>MSCGNAKINSPAPSFEEVALMPNGSFKKISLSSYKGKWVVLFFYPLDFTFVCPTEVIAFSDSVSRFNELNCEVLACSIDSEYAHLQWTLQDRKKGGLGTMAIPILADKTKNIARSYGVLEESQGVAYRGLFIIDPHGMLRQITVNDMPVGRSVEEVLRLLEAFQFVEKHGEVCPANWKKGDPGMKPEPNASVEGYFSKQ[5x]

T(SH)2 participates in crucial thiol-disulfide exchange reactions and serves as electron donor in the reduction of hydrogen peroxide to water catalyzed by the tryparedoxin/tryparedoxin peroxidase couple (TXN/TXNPx). Leishmania major TXNPx (LmTXNPx) is an obligate homodimer whose active site is formed by the N-proximal peroxidatic cysteine (Cp) from one subunit and a C-proximal resolving cysteine from the two-fold symmetry related subunit (Cr′)89. In the first reaction, oxidized TXNPx binds TXN, which reduces the inter-subunit disulfide bridge (Cp–Cr′) and, thereafter, is reduced by T(SH)2. In the second reaction, the Cp thiolate of a TXNPx monomer reduces the hydrogen peroxide to water and is oxidized to sulfenic acid (-SOH); the sulfenic Cp then reacts with the Cr′ of the two-fold symmetry related monomer forming a disulfide bridge.

In this paper, we report the X-ray crystal structure of LmTXNPx in FF conformation at high resolution. The overall structure of LmTXNPx-FF is very similar to that of LmTXNPx-LU. Both quaternary structures are pentamers of dimers assembled to form a toroidal ring with an outer diameter of 120 Å and an internal diameter of about 60 Å. Optimal structure superimposition between LmTXNPx-FF and LmTXNPx-LU highlights that conformational changes occur just in two regions: the 43–53 loop containing Cp (Cys52) and the C-terminal tail (residues 169–199) containing Cr′ (Cys173′). In LmTXNPx-FF Cp is part of the first turn of an α-helix, located in a narrow solvent-accessible pocket that constitutes the active site. Cp is hydrogen bonded to the highly conserved Thr49 and Arg128 residues, both of which are essential for catalysis. The C-terminal tail (residues 169–199), which is missing in LmTXNPx-LU, is completely visible in LmTXNPx-FF, thus revealing the complete active site structure of the protein. Cr′ is part of a loop and its side chain is embedded in a hydrophobic cavity formed by the 170–187 residues. The entrance to this active site cavity is covered by the short C-terminal α-helix (residues 187–195), which protects Cr′ from over-oxidation. Reduced LmTXNPx-FF is ready to exert its catalytic function, i.e., reduction of hydrogen peroxide to water, involving oxidation of Cp to sulphenic acid.>[2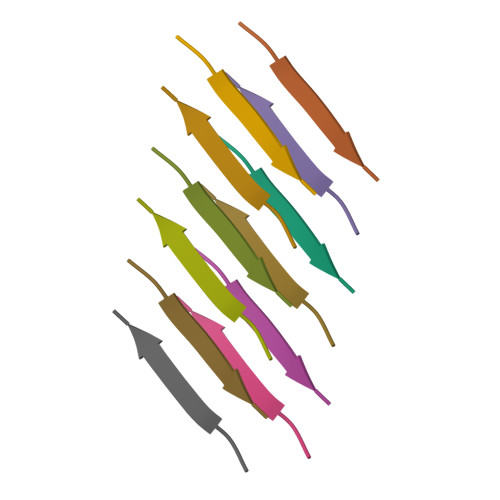x]NFGAILS>KSDSENIKDVKLQLNYAYEIIPVDYTNCNIDYLTTHDFYIDISSYKKKNFSVDSEVESYITTKFTKNQKVNIFGLPYIFTRYDVYYIYGGVTPSVNSNSENSKIVGNLLIDGVQQKTLINPIKIDKPIFTIQEFDFKIRQYLMQTYKIYDP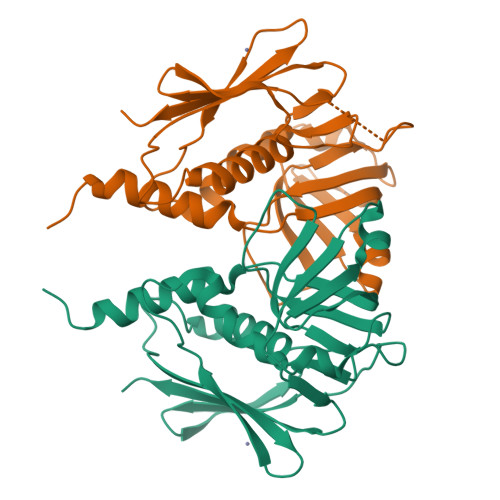NSPYIKGQLEIAINGNKHESFNLYDATSSSTRSDIFKKYKDNKTINMKDFSHFDIYLWTK[3x]N-(4-chlorophenyl)-N'-[(2R)-1-hydroxybutan-2-yl]urea 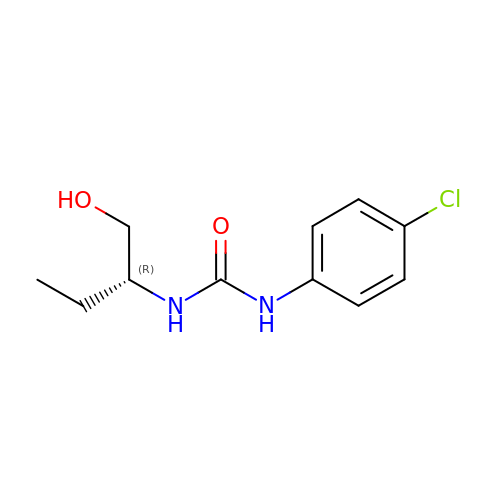| C11 H15 Cl N2 O2 | WLAQZHZJODLWGO-SECBINFHSA-N>LMGDDKVKKEVGRASWKYFHTLLARFPDEPTPEEREKLHTFIGLYAELYPCGECSYHFVKLIEKYPVQTSSRTAAAMWGCHIHNKVNEY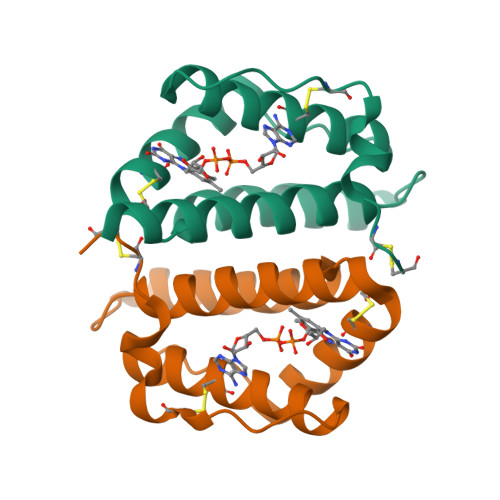LKKDIYDCATILEDYDCGCSDSDGKRVS[2x]> SMSEQSICQARAAVMVYDDANKKWVPAGGSTGFSRVHIYHHTGNNTFRVVGRKIQDHQVVINCAIPKGLKYNQATQTFHQWRDARQVYGLNFGSKEDANVFASAMMHALEV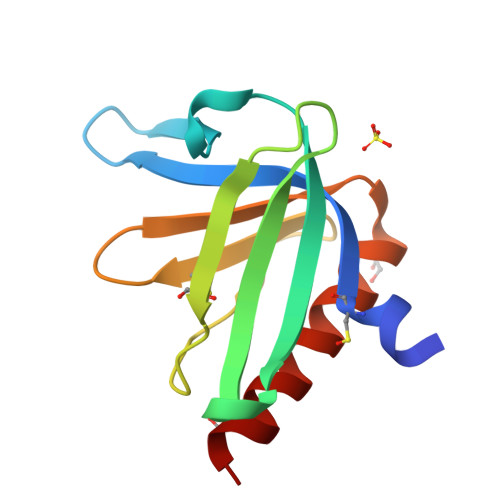LNS;> EHIPPPPRPP> ETGNYMGNPWTEYMAKYDIEEVHGSGIRVDLGEDAEVAGTQYRLPSGKCPVFGKGIIIENSNTAFLTPVATGNQYLKDGGFAFPPTEPLMSPMTLDEMRHFYKDNKYVKNLDELTLCSRHAGNMIPDNDKNSNYKYPAVYDDKDKKCHILYIAAQENNGGGGGSGSDITQQAKDIGAGPVASCFTTRMSPPQQICLNSVV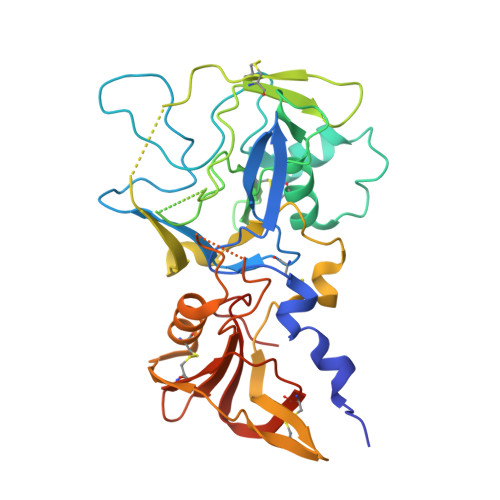NTALSGGSGMFCFRPAKDISFQNYAYLSKNVVDNWEKVCPRKNLQNAKFGLWVDGNCEDIPHVNEFPAIDLFECNKLVFELSASDQPGGSGYKSHGKGYNWGNYNTETQKCEIFNVKPTCLINNAAYIATTALSHPIEVEGTKHHHHHH>MGSDKIHHHHHHMAFFDLPLEELKKYRPERYEEKDFDEFWEETLAESEKFPLDPVFERMESHLKTVEAYDVTFSGYRGQRIKGWLLVPKLEEEKLPCVVQYIGYNGGRGFPHDWLFWPSMGYICFVMDTRGQGSGWLKGDTPDYPEGPVDPQYPGFMTRGILDPRTYYYRRVFTDAVRAVEAAASFPQVDQERIVIAGGSQGGGIALAVSALSKKAKALLCDVPFLCHFRRAVQLVDTHPYAEITNFLKTHRDKEEIVFRTLSYFDGVNFAARAKIPALFSVGLMDNICPPSTVFAAYNYYAGPKEIRIYPYNNHEGGGSFQAVEQ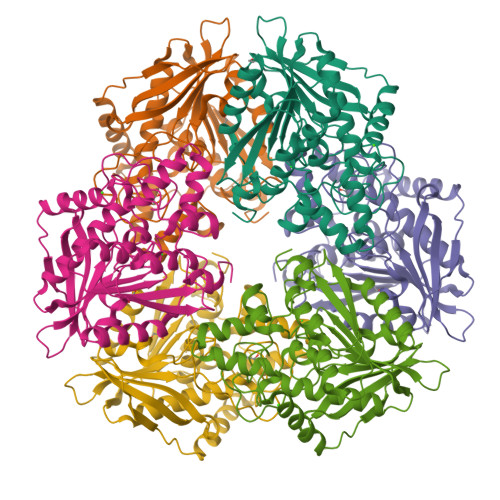VKFLKKLFEKG[6x]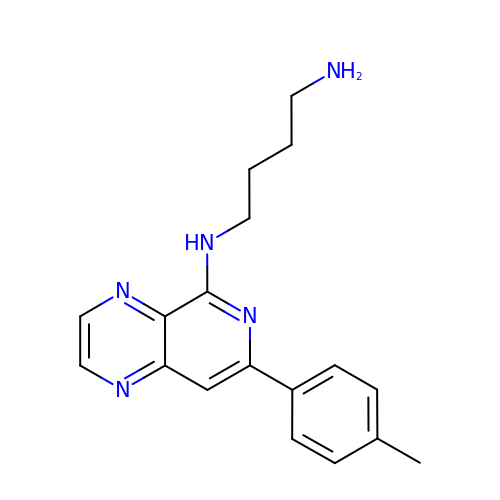~{N}'-[7-(4-methylphenyl)pyrido[3,4-b]pyrazin-5-yl]butane-1,4-diamine | C18 H21 N5 | FYJFZOONLWHKMF-UHFFFAOYSA-N[[2-[(2~{R},3~{S},4~{R},5~{R})-5-(6-aminopurin-9-yl)-3,4-bis(oxidanyl)oxolan-2-yl]ethylamino]-azanyl-methylidene]azanium | C12 H19 N8 O3 | 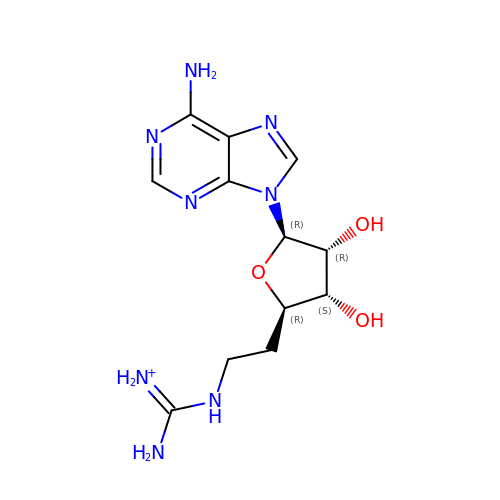OIGRVZYOOMUALG-IOSLPCCCSA-O> SSQIRQNYSTDVEAAVNSLVNLYLQASYTYLSLGFYFDRDDVALEGVSHFFRELAEEKREGYERLLKMQN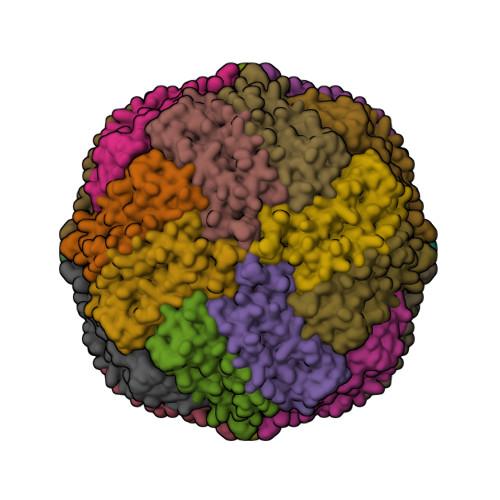QRGGRALFQDIKKPAEDEWGKTPDAMKAAMALEKKLNQALLDLHALGSARTDPHLCDFLETHFLDEEVKLIKKMGDHLTNLHRLGGPEAGLGEYLFERLTLKHD Silodosin 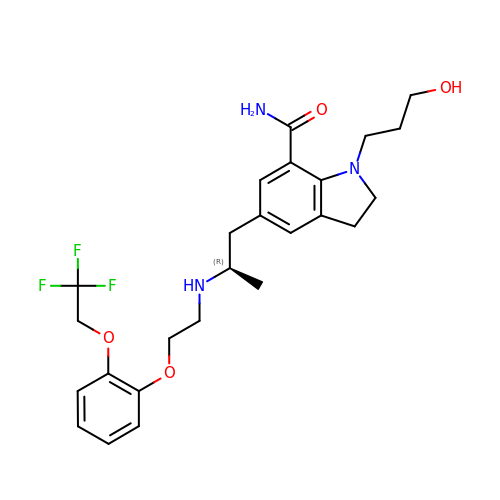| C25 H32 F3 N3 O4 | PNCPYILNMDWPEY-QGZVFWFLSA-N> MSKTDYILRALSKISHKRWEHYIINRVVHTLDDPDIEFVCQQCIRKEGHLGKIYLADLLFPQLNLYLEIDEAHHDSNDARKADAVRRLDIVEATGFQEERIPASNITLSEVNKLVDEFVRLVKDKKEELENQGLFFRWDYDERYSAKKHINTGYMAVGPNSVFRYHRDALQCFGYRREGHHQSGGWALPAEVAQSIGLTGRVMVWFPRLYEAGEWKNALSADGNKITEQSLNATRNYQETWDYRIVMAHSRDELNRTLYRFLGVFAIDVDKSSDEVKVFSRVYSRVNVYRSQN

PvuRts1I is a modification-dependent endonuclease with high selectivity for 5-hydroxymethyl­cytosine over 5-methylcytosine and cytosine. PvuRts1I family enzymes are classified as bacterial type IV modification-dependent restriction endonucleases and they are known to play an important role in defence against phage infection. In contrast, most enzymes of the PvuRts1I family selectively bind to 5-hmC and 5-glucosylated methylcytosine (5-gmC) with high specificity over both 5-mC and cytosine, and cleave substrate DNA at a fixed distance from the modified cytosine. The structure consists of two domains: a novel SRA-like domain that recognizes 5-hmC and an unusual nuclease domain that has not previously been curated by the NCBI Conserved Domain Database.

The PvuRts1I crystals diffracted to 2.9 Å resolution and phases were obtained by the single-wavelength anomalous dispersion (SAD) method. However, part of the putative active site (amino-acid residues 71–76) was not visible in the electron-density map and could not be modelled, and may be highly flexible in the absence of the DNA substrate. A search of the protein-structure database using DALI revealed that the overall structure of the N-terminal domain is similar to the very short patch repair (Vsr) endonuclease, with a root-mean-square deviation (r.m.s.d.) of 2.4 Å. Comparison with structures in the PDB using the DALI server revealed that the C-terminal DNA-binding domain of PvuRts1I is related to 5-mC/5-hmC binding modules, including the SRA domains of Arabidopsis SUVH5 (Z-score = 4.9; r.m.s.d. = 3.1 Å) and human UHRF1 (Z-score = 4.4; r.m.s.d. = 3.1 Å) and the SRA-like domain of another modification-dependent restriction endonuclease MspJI (Z-score = 4.2; r.m.s.d. = 3.2 Å). As for other 5-mC/5-hmC binding modules, the overall shape of the SRA-like domain of PvuRts1I resembles a saddle, with a concave surface at the open side of the β-barrel. Similarly, we speculate that PvuRts1I recognizes 5-hmC using this surface. The interaction interface between the two molecules is formed by helices α1 and α2 of each subunit, and involves hydrophobic interactions and hydrogen bonds. The buried surface area of the interface is approximately 812 Å2, which is clearly adequate to stabilize the dimer in solution. The recognition sequence of PvuRts1I is approximately 22 bp long and 74 Å in length, which fits well with the distance between the two recognition sites in the dimeric PvuRts1I assembly. The binding pocket of PvuRts1I is shallower and wider than that in SUVH5 and UHRF1.2-{8-fluoro-2-[2-(hydroxymethyl)-3-(1-methyl-5-{[5-(4-methylpiperazin-1-yl)pyridin-2-yl]amino}-6-oxo-1,6-dihydropyridin-3-yl)phenyl]-1-oxo-1,2,3,4-tetrahydroisoquinolin-6-yl}-2-methylpropanenitrile 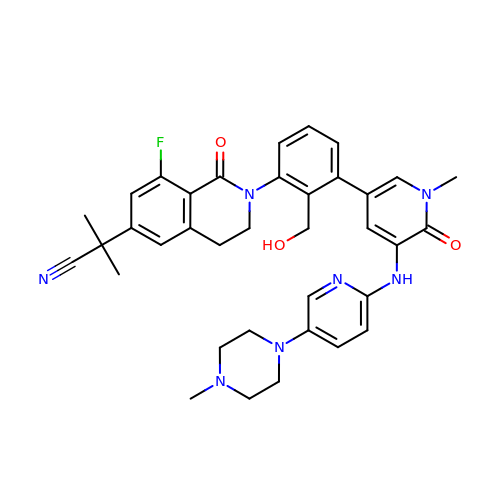| C36 H38 F N7 O3 | AGMLIXLHTZGRPZ-UHFFFAOYSA-N imidazolidin-2-one 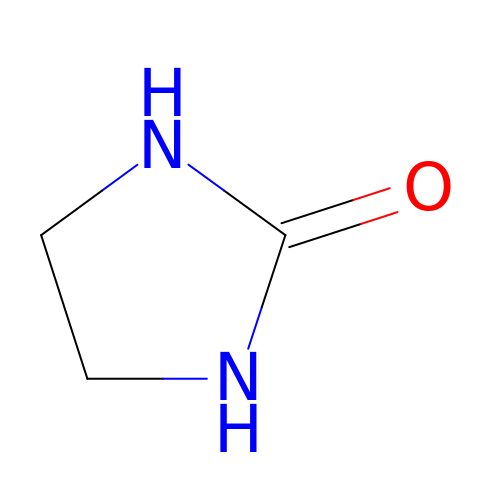| C3 H6 N2 O | YAMHXTCMCPHKLN-UHFFFAOYSA-N>GEFEKLEALEQLQSHIEGWEGSNLTDICTQLLLQGTLLKISAGNIQERAFFLFDNLLVYCKRKSRVTGSKKSTKRTKSINGSLYIFRGRINTEVMEVENVEDGTADYHSNGYTVTNGWKIHNTAKNKWF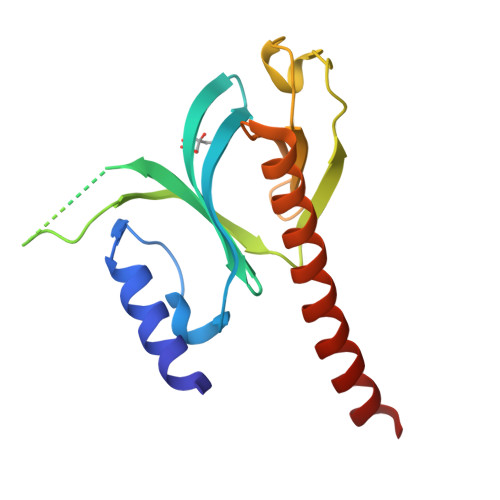VCMAKTAEEKQKWLDAIIREREQRESLKLGMERDAYVM[2x]>[2x]AHHHHNSGPLEFTVSANTNPATDAVRESILANPGFGKYYTDHMVSIDYTVDEGWHNAQVIPYGPIQLDPSAIVLHYGQEIFEGLKAYRWADGSIVSFRPEANAARLQSSARRLAIPELPEEVFIESL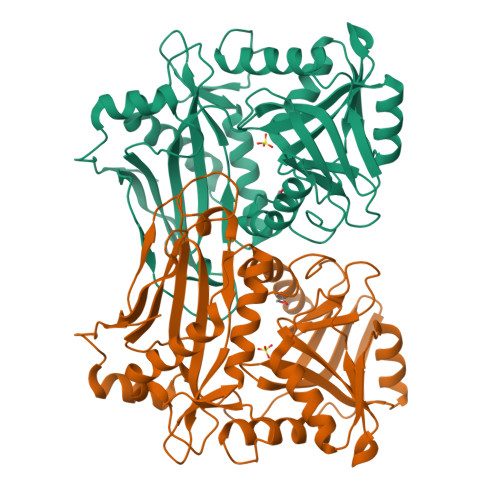RQLIAVDEKWVPPAGGEESLYLRPFVIATEPGLGVRPSNEYRYLLIASPAGAYFKGGIKPVSVWLSHEYVRASPGGTGAAKFGGNYAASLLAQAQAAEMGCDQVVWLDAIERRYVEEMGGMNLFFVFGSGGSARLVTPELSGSLLPGITRDSLLQLATDAGFAVEERKIDVDEWQKKAGAGEITEVFACGTAAVITPVSHVKHHDGEFTIADGQPGEITMALRDTLTGIQRGTFADTHGWMARLN> TQVFDLEGYGAISRAMGGTSSSYYTGNAALISNPATLSFAPDGNQFELGLDVVTTDIKVHDSHGAEAKSSTYAVGAQLSYVAQLDDWRFGAGLFVSSGLGTEYGSKSFLSQTENGIQTSFDNSSRLIVLRAPIGFSYQATSKLTFGASVDLVWTSLNLELLLPSSQVGALTAQGNLSGGLVPSLAGFVGTGGAAHFSLSRNSTAGGAVDAVGWGGRLGLTYKLTDNTVLGAMYNFKTSVGDLEGKATLSAISGDGAVLPLDGDIRVKNFEMPASLTLGLAHQFNERWVVAADIKRAYWGDVMDSMNVAFISQLGGIDVALPHRYQDITVASIGTAYKYNNDLTLRAGYSYAQQALDSELILPVIPAYLKRHVTFGGEYDFDKDSRINLAISFGLRERVQTPSYLAGTEMLRQSH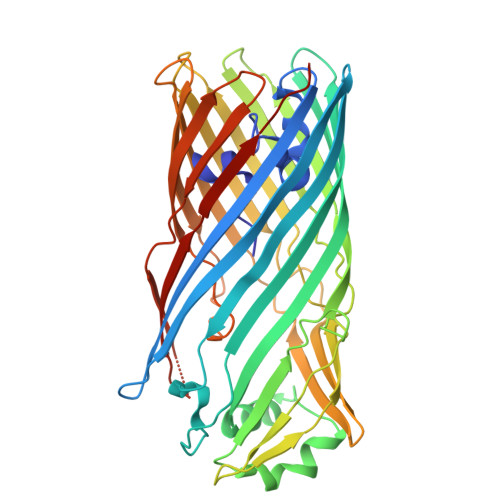SQINAVVSYSKNFHHHHHH>[2x]AGGGTT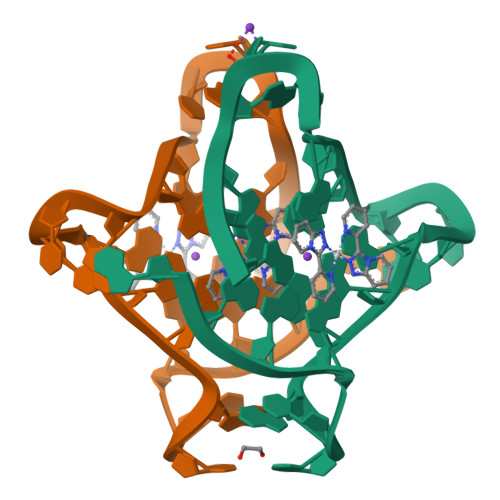AGGGTTAGGGTTAGGG> MGRFIFVSFGLLVVFLSLSGTGADCPSGWSSYEGHCYKPFNEPKNWADAERFCKLQPKHSHLVSFQSAEEADFVVKLTRPRLKANLVWMGLSNIWHGCNWQWSDGARLNYKDWQEQSE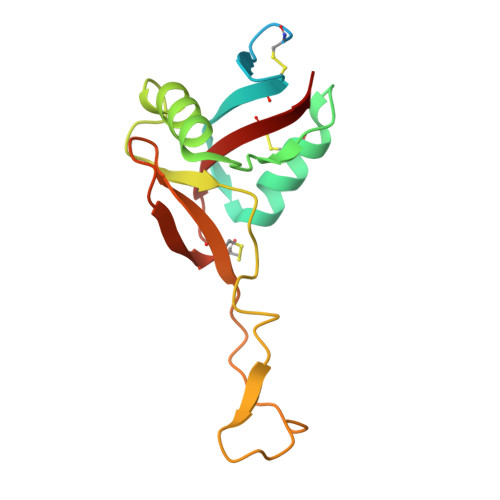CLAFRGVHTEWLNMDCSSTCSFVCKFKA> HHHHHHSSGLVPRGSHMMRSVYPLARRSMAAYTMHNMTVPEPYDYLEDPENPETKTFVNEQNAFFEEYFASEAELRKKIFESISNSQDYPRTSNPSYINGHYYYYHNSGLQNQSVLMRAMSLTDTAPSIFLDPNSMSSDGTTALKATAWSEDESMLAYSLSDKGSDWQRIHVRRADTVEDTSDVIEWAKFTAIAWWHNLGFFYTRYPALQGDVDKGAETDAAQDAFICFHRIGRPQDEDVVILSVPEHPQWNMGASVSDCHSYVIVVLFDGCEPHNLVWVAELPSVEKGLGSEPLVFKKLVNEFAGRYTYLGNEGSTFYFVTTRDAPRKKIVSIDIHTGQETVIVEQQRSVLSQAALVKKTLLLAYLEDVKDVFYYCRLEDPTLNAIPLPIGTITSFFSDRKKDFVSFKITSFLLPGRSFFLDINDPQSSLRVFKDDTVEGLLVDDFVTEQTFYNSSDGVRIPMFIVYRKGSVSSESPLLLYGYGGFNIPLTPAFSSSRMVFLRDLGGVLAVLNIRGGGEYGEEWHDAGRRACKQNCFTDFIEGAKFLHRQGYGSPQTTAIMGGSNGGLLVAAVANQAPELFRCVVCRVGVLDMYKFHKFTIGHAWKSDYGDPEKEEDFRVLQQYSPLHNIKSGIKYPAILVVTGDHDDRVVPLHSLKYVATLQHMNPNEGGPFLARIEVAAGHGAGKPTSKILREAGDIYTFIAKNINASWKE

Amidst these challenges, a member of the endopeptidase enzyme family, T. cruzi 80 kDa prolyl-oligopeptidase (TcPOP, enzyme ID EC 3.4.21.26), has been identified as a potential vaccine target for Chagas disease. It degrades collagen and fibronectin extracellular matrix components on host cells, facilitating parasite invasion. Our cryo-EM data confirm that TcPOP comprises two distinct domains: a catalytic α/β-hydrolase domain, which houses the active site featuring the catalytic triad, and a β-propeller domain, which likely regulates substrate access. The spatial arrangement of these domains reveals a cylindrical structure, with the β-propeller domain capping the catalytic α/β-hydrolase domain, as previously postulated.

Here we report the three-dimensional structure of TcPOP in open and closed conformation, at a global resolution of 3.8 and 3.6 Å, respectively, determined using single-particle cryo-electron microscopy. The initial data collection, comprised of 20,080 micrographs, revealed severe preferential orientation, resulting in poor map reconstructions. We therefore tilted the grids to 30° and 35° to increase the number of views visualised in the electron micrographs. This significantly improved the number of views, and the resulting map was drastically improved with continuous density and minimal anisotropic features. 3D classification revealed two distinct conformations of TcPOP i.e., open and closed, indicating intrinsic conformational heterogeneity of the dataset. Two conformations of TcPOP could be easily identified in 3D classification, spanning from fully closed to fully open with an overall motion of ~22° between the two domains. The evident stability of the α/β hydrolase domain observed in both open and closed conformations, as well as in those from aligned cryo-EM maps, suggests possible regions that are exposed to the immune system when the enzyme is secreted in the blood, and therefore likely to include potential epitopes. Our data show that TcPOP clearly fluctuates between open and closed states independently from the presence of the substrate, confirming that the observed open and closed conformations occur in solution and are observed without the usage of any additive. Taken together, our HDX-MS data corroborate with the existence of the TcPOP open and closed conformations that could be resolved in cryo-EM, and with the presence of intermediate conformations that arise from the switching of selected helices and loops at different rates.>GMKYDIPTMTAEAVSLLKSLISIPSISREETQAADFLQNYIEAEGMQTGRKGNNVWCLSPMFDLKKPTILLNSHIDTVKPVNGWRKDPFTPREENGKLYGLGSNDAGASVVSLLQVFLQLCRTSQNYNLIYLASCEEEVSGKEGIESVLPGLPPVSFAIVGEPTEMQPAIAEKGLMVLDVTATGKAGHAARDEGDNAIYKVLNDIAWFRDYRFEKESPLLGPVKMSVTVINAGTQHNVVPDKCTFVVDIRSN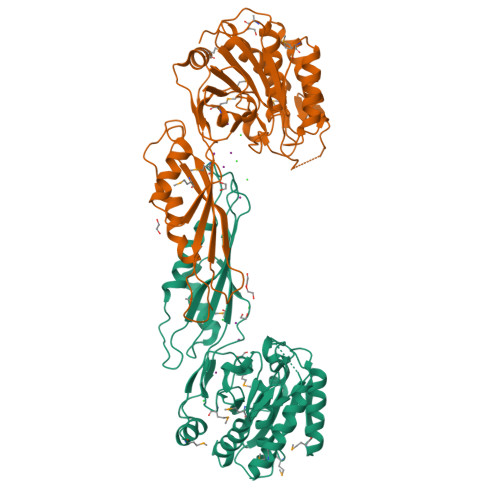ELYSNEDLFAEIRKHIACDAKARSFRLNSSRIDEKHPFVQKAVKMGRIPFGSPTLSDQALMSFASVKIGPGRSSRSHTAEEYIMLKEIEEAIGIYLDLLDGLKL[2x]> LRYTTEIIKCPQPKTLDEFTIIQ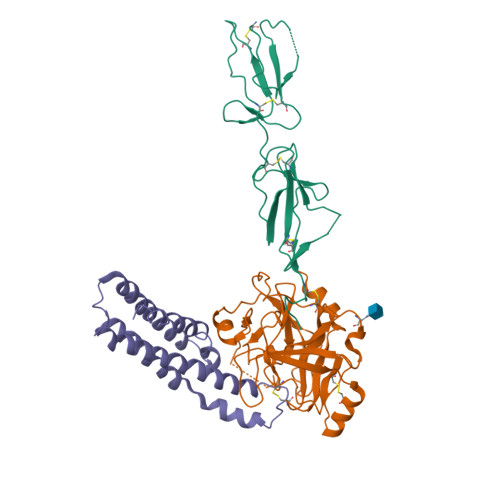NLQPQYQFRDYFIATCKQGYQLIEGNQVLHSFTAVCQDDGTWHRAMPRCKIKDCGQPRNLPNGDFRYTTTMGVNTYKARIQYYCHEPYYKMQTRAGSRESEQGVYTCTAQGIWKNEQKGEKIPRCLPVCGKPVNPVEQRQR;> IIGGQKAKMGNFPWQVFTNIHGRGGGALLGDRWILTAAHTLYPKEHEAQSNASLDVFLGHTNVEELMKLGNHPIRRVSVHPDYRQDESYNFEGDIALLELENSVTLGPNLLPICLPDNDTFYDLGLMGYVSGFGVMEEKIAHDLRFVRLPVANPQACENWLRGKNRMDVFSQNMFCAGHPSLKQDACQGDSGGVFAVRDPNTDRWVATGIVSWGIGCSRGYGFYTKVLNYVDWIKKEMEEED;> GSTGSSNRYQSYLEGVKYNVDSAIQTITKIYNTYTLFSTKLTQMYSTRLDNFAKAKAKEEAAKFTKEDLEKNFKTLLNYIQVSVKTAANFVYINDTHAKRKLENIEAEIKTLIAKIKEQSNLYEAYKAIVTSILLMRDSLKEVQGIID Given the auxotrophic nature of pneumococci for certain amino acids, the Ami ABC transporter system, orchestrating oligopeptide uptake, becomes indispensable in host compartments lacking amino acids. The system comprises five exposed Oligopeptide Binding Proteins (OBPs) and four proteins building the ABC transporter channel. Crucially, SBPs determine the specificity of their respective transport systems, thereby governing the range of molecules capable of entering the cell. The five lipoproteins exhibit pairwise sequence identity of ~52–60% and share a very similar overall folding.

One such peptide, FPPQSV (peptide 1), derived from Prevotella species, has been shown to induce significant changes in gene expression and enhanced colonization when bound by AliD. Hence, peptides bind to OBPs, however, peptide-binding occurs with a low affinity when both, the fluorescently labelled AliD and the peptides as ligand are in solution and binding experiments are conducted at 25° C. The crystal structure of the AliD:peptide 1 complex was obtained by co-crystallization at 2.18 Å resolution. The asymmetric unit contained two monomers (chains A and B) with virtually identical structures (rmsd of 0.14 Å for 564 Cα atoms superposition). In these structures, AliD monomers adopt a closed conformation, resulting in a complete engulfment of peptide 1 between the two protein lobes without contact with the bulk solvent. The ligand-bound and unbound forms of AliD retained the three-dimensional structures of the individual domains unaltered, as both conformations were related by a rigid-body rotation of ~20° of Lobe 1 (Domain III) relative to Lobe 2 (Domains I and III). Specifically, the side chain of the initial substrate residue (F) finds accommodation within a hydrophobic pocket cavity, designated as P1. The amine N-terminal tip of the oligopeptide substrate establishes electrostatic interactions with residue D501 and forms H-bonds with the main-chain atoms of residue V499, both from Domain III. Moreover, residues located in Domain I of AliD including G39, A52, D53 and N608 (located in pockets P4 and P5), actively contribute to stabilizing the substrate through polar interactions. These polar interactions are complemented by several hydrophobic interactions facilitated by aromatic residues such as Y50, Y51, W498, F481, F518 and Y519 (located in pockets P1-P3), resulting in the tight binding of the initial five residues of peptide 1 to the AliD protein. In contrast, the ultimate residue of peptide 1 demonstrate fewer interactions with the OBP. Consistently, we observed an increase in the B-factors of the substrate from the N- to C-terminus, along with the presence of two different conformations for the sixth residue in the substrate.

>[2x]ASSDTKTYSSTFSGNPTTFNYLLDYYADNTAIITNLVDGLLENDNHGNLVPSLAEDWSVSSDGLTYTYKLRKDAKWFTADGEEYSPVKAQDFVTGIKYAVDNKSQAIDLIQNSIKGLNDYITGADSDFSKVGVKAIDDQTVEYTLARPEPYWNSKTTNSILFPVNEEFLNSKGKDFGTLSPDSILYSGPYLLKDFTSKSSIEYVKNPHYYDHDKVSIEHVKLAYFDGSDQELTIRNFESGAYSIAGVYPNSSNFAKTKEKYKDNIVYSLQDKTSWYFNFNVNRKAYNHTSKTTDEQKKSTETAVLNKNFRQAVNFALDRTAYSAQSNGEEAASKTLLNTLVPPTFVQVGDKTFGEVVASKLVNYGTEWSGINLADAQDAYFNKEKAQAKFAEAKKELTSQGVTFPIHLDVAVDQTSKNAVTGMNSVKQTLESVLGSDNIVIDVQQLSTDDFNNVAFLAPTAADRDYDFNFDGWVGDYQDPSTYLNPFNAEDGFYLKIFGLDAKEDKEKITSLGLDTYTKMLKDADRENKDVAKRYEKYAEAQAWMIDNSLIMSAMSSGGTASVTKVTPFTRGYSLVGIKGDGNNYKYMKLQKDTVTTKQFEEAKSKWEQESKKAIEKAQKEAEKHVK;>[2x]FPPQSV>ANFTCAVASGTTCKSAILYTSPNATTYGNLVARFNTTTLPDLLGANGLPDGTLSSAPVAANSTVKIPFRCRCNGDVGQSDRLPIYVVQPQDGLDAIARNVFNAFVTYQEIAAANNIPDPNKINVSQTLWIPLPCSCDKEEGSNVMHLAYSVG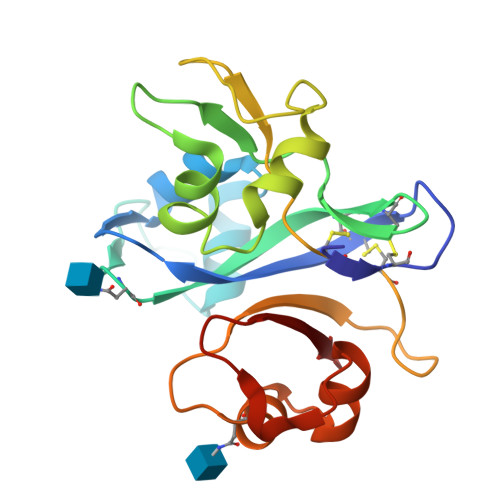KGENTSAIAAKYGVTESTLLTRNKIDDPTKLQMGQILDVPLPV[3x]>MNKPSFLLVGLLVVSGVLGAAETKVKYPDGFRSWYHVKSMVIQPGHPLENPFGGIHHVYANAEAIQGLRGGNYPDGAVLVVDLFDYQEDNHALVEGKRKLIGVMERDAKRFSATGGWGYEGFGEGKPDKRLVTDGGQGCFGCHAAQKESQYVFSRLRD[2x]

Cytochromes c′ (cyts c′) are a group of putative NO-binding heme proteins that fall into two families: the well-characterized four alpha helix bundle fold (cyts c′-α) and an unrelated family with a large beta-sheet fold (cyts c′-β) resembling that of cytochromes P460. Of these, cytochrome P460 (cytP460) is a heme enzyme that oxidizes hydroxylamine to N2O as part of nitrification (1), whereas the evolutionarily related cytochrome c′-β (cyt c′-β) binds the diatomic gases, NO and CO (2). By contrast, our recent crystal structure of cyt c′-β from Methylococcus capsulatus (Bath) (McCP-β) reveals a hydrophobic distal pocket dominated by two Phe residues (F32 and F61), a structural feature we have named the “Phe cap. Proposed roles for cyt c′-β proteins include protection against NO stress generated during nitrification.

The F61V variant exhibits Fe–C distances of 2.01 and 2.00 Å and a similar bent geometry to the native ligand–bound structure with Fe–C–O angles of 166° and 177° for monomer A and B, respectively. The F61V variant still displays two possible conformations of Phe 32 in the presence of CO. Similar to the wt Fe(II)CO complex, two orientations of Phe 32 can be seen in the F61V crystal structure. However, unlike the wt structure, where a unique Phe 32 orientation was seen in each monomer, F61V displays two orientations in both monomers. RR measurements of F61V and F32V Fe(II)CO complexes support our hypothesis that the local negative polarity of the Phe 32 aromatic quadrupole limits buildup of charge associated with Fe(II)→CO(π∗) backbonding, thereby weakening the Fe–CO bond. The pair of ν(FeCO) frequencies observed for the F61V variant (483 and 495 cm−1) are similar to those of the ν(FeCO) doublet for wt McCP-β (481 and 491 cm−1), with the lower frequency ascribed to CO interacting with the local negative polarity of the aromatic quadrupole of Phe 32. In line with RR data that indicate a modest weakening of the Fe–CO bond (because of the Phe 32 aromatic quadrupole), the CO off rates of wt and F61V are 1.5 (±0.2)-fold and 2.5 (±0.3)-fold higher than that of F32V. Crystallographic and RR data confirm that NO and CO ligands interact with the Phe 32 ring face in the F61V variant but are unaffected by any aromatic quadrupole in the F32V variant.>MAHHHHHHSGMSGMRVYLGADHAGYELKQRIIEHLKQTGHEPIDCGALRYDADDDYPAFCIAAATRTVADPGSLGIVLGGSGNGEQIAANKVPGARCALAWSVQTAALAREHNNAQLIGIGGRMHTV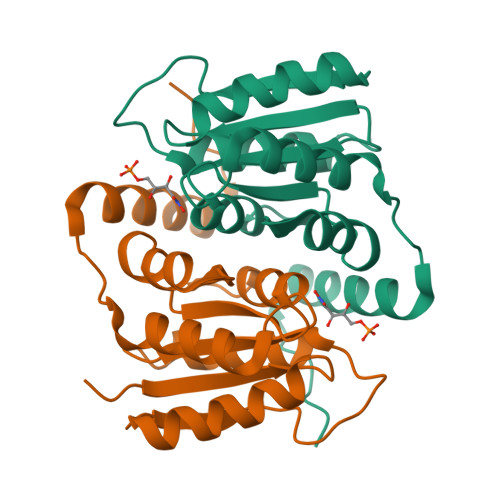AEALAIVDAFVTTPWSKAQRHQRRIDILAEYERTHEAPPVPGAPA[5x]> ASWSHPQFEKGAELPAQKWWHTGALYRIGDLQAFQGHGAGNLAGLKGRLDYLSSLKVKGLVLGPIHKNQKDDVAQTDLLQIDPNFGSKEDFDSLLQSAKKKSIRVILDLTPNYRGENSWFSTQVDTVATKVKDALEFWLQAGVDGFQVRDIENLKDASSFLAEWQNITKGFSEDRLLIAGTNSSDLQQILSLLESNKDLLLTSSYLSDSGSTGEHTKSLVTQYLNATGNRWCSWSLSQARLLTSFLPAQLLRLYQLMLFTLPGTPVFSYGDEIGLDAAALPGQPMEAPVMLWDESSFPDIP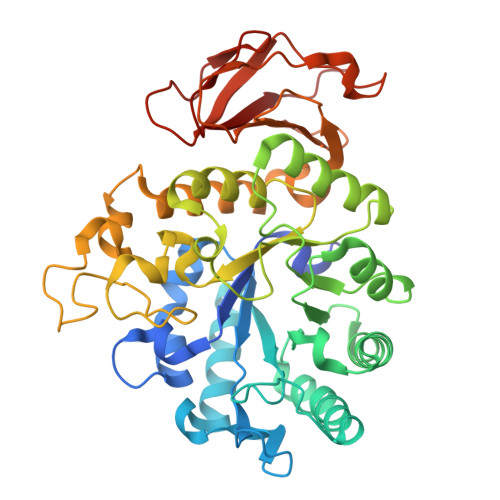GAVSANMTVKGQSEDPGSLLSLFRRLSDQRSKERSLLHGDFHAFSAGPGLFSYIRHWDQNERFLVVLNFGDVGLSAGLQASDLPASASLPAKADLLLSTQPGREEGSPLELERLKLEPHEGLLLRFPYAA5-[(2,3-Dihydro-1H-inden-5-yloxy)methyl]-2-furoic 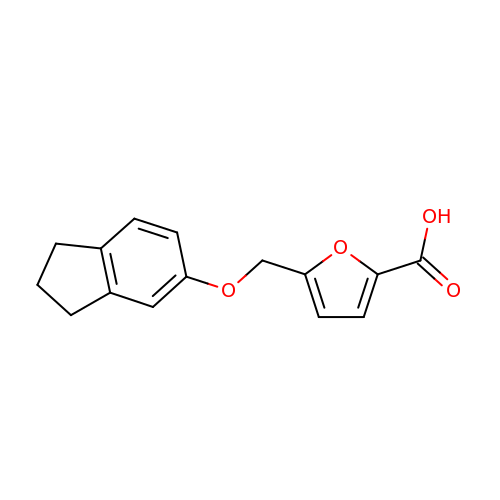acid | C15 H14 O4 | BQKLXOGKDTYPRT-UHFFFAOYSA-N>[2x]MARSNLLRD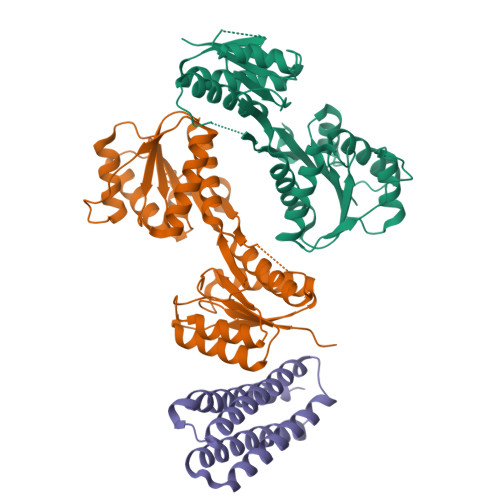KKVEKEPIKPKIVLISHIKTNPYWLDIKAGAERAAKERGAVVEFLGPTTASTEDGLKLFDMATSAKVSGIITYVQEEGQYKKKINSAMEKGIPVVTIASDEEDSNRIAYVGTDNVLAGQVAGKEMVKQIGTSGNVAIVMGGKNVKNQKERVEGFTQYIKSNSNLKIVDTDSSDAMLLEAEIITRKILNRNDNINALFCTSALDGIGAARAVKDLNYKDRVKIICFDDLDDTLSNIRNGLVSATIVQKSNEMGYRAVNIIMDKIEGKSNKFSKSLIDVNVINKSDVDSYKRGDDKVEN;> MGSSHHHHHHQGSMLNNMLITNEIKQHVDSSLDNFNQYILNGTPSKKESYNNEVILAKQKIGNLKKNSDDVNQYILRDLDNTLDSYIESSKNTISAYENKEGYVFYYDDFVAAKNIASYCDAYASTLMQNFLEANSIAYKELNRNSS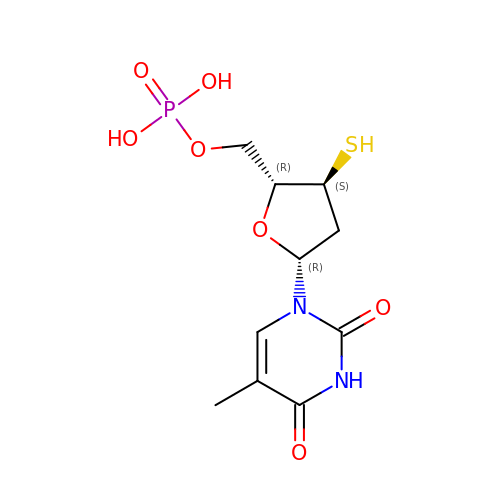3'-THIO-THYMIDINE-5'-PHOSPHATE | C10 H15 N2 O7 P S | BORVFKJZAOEGOO-GJMOJQLCSA-N The IM component LptB2FG comprises an ATP-binding cassette (ABC) transporter, which powers the transport of LPS across the bridge. The cytoplasmic LptB dimer binds and hydrolyses ATP and the transmembrane (TM) domains of LptF and LptG create a cavity to accommodate LPS. LptB2 constitutes the cytoplasmic NBD dimer and the six TM helices of LptF and LptG (F_TM1-TM6 and G_TM1-TM6) constitute two TMDs that are arranged to form a central cavity with two surface gaps between TM1F and TM5G and TM1G and TM5F termed as lateral gates. To understand the mechanisms of how LptB2FGC recognises and acts to transport LPS, we obtained high-resolution cryo-electron microscopy (cryo-EM) structures of LptB2FGC complexed with substrate LPS or ATP analogue β-γ-imidoadenosine 5′-triphosphate (AMP-PNP).

The cryo-EM structure of sfLptB2FGC was determined to 3.1 Å resolution. However, due to possible flexibility, we are unable to see clear density for the periplasmic domain of LptC. In our structure, residues M1, R5, I9, L12, V16, M19 and N23 from the TM helix of LptC interact with residues Q293, L300, L305, L304, L307, L311 and T314 from the TM5 of LptF, respectively. In contrast, only G21 from the TM helix of LptC interacts with V36 of TM1 of LptG. Comparing to the sfLptB2FG LPS-bound structure, the presence of the TM helix of LptC makes the lateral gate TM1G/TM5F of sfLptB2FGC structure much widely opened, along with the neighbouring TM2 and TM3 of LptG and TM4 and TM6 of LptF moved outward, resulting an enlarged central cavity. In contrast to the two recent publications, a density for LPS is identified in the cavity of sfLptB2FGC with all features visible as in the sfLptB2FG structure except the inner core of the LPS. Interestingly, the LPS molecule trapped in the cavity of sfLptB2FGC is about 7.3 Å away from that of sfLptB2FG structure referring to the position of the 1′-phosphate group. The LPS molecule in the sfLptB2FGC structure positions in proximity to LptG with kinked acyl tails rather than drooped as seen in the sfLptB2FG structure. In the cavity of sfLptB2FGC, we can also see that hydrophobic residues L17 and M24 from the TM helix of LptC interact with the bound LPS, suggesting that the TM helix of LptC is also involved in LPS recognition. The number of residues from the TM helices of LptF and LptG that have been shown to interact with LPS in the enlarged cavity of sfLptB2FGC are greatly reduced compared to the structure of sfLptB2FG.

>[2x]MATLTAKNLAKAYKGRRVVEDVSLTVNSGEIVGLLGPNGAGKTTTFYMVVGIVPRDAGNIIIDDDDISLLPLHARARRGIGYLPQEASIFRRLSVYDNLMAVLQIRDDLSAEQREDRANELMEEFHIEHLRDSMGQSLSGGERRRVEIARALAANPKFILLDEPFAGVDPISVIDIKRIIEHLRDSGLGVLITDHNVRETLAVCERAYIVSQGHLIAHGTPTEILQDEHVKRVYLGEDFRL;> MSKARRWVIIVLSLAVLVMIGINMAEKDDTAQVVVNNNDPTYKSEHTDTLVYNPEGALSYRLIAQHVEYYSDQAVSWFTQPVLTTFDKDKIPTWSVKADKAKLTNDRMLYLYGHVEVNALVPDSQLRRITTDNAQINLVTQDVTSEDLVTLYGTTFNSSGLKMRGNLRSKNAELIEKVRTSYEIQNKQTQP;> MIIIRYLVRETLKSQLAILFILLLIFFCQKLVRILGAAVDGDIPANLVLSLLGLGVPEMAQLILPLSLFLGLLMTLGKLYTESEITVMHACGLSKAVLVKAAMILAVFTAIVAAVNVMWAGPWSSRHQDEVLAEAKANPGMAALAQGQFQQATNGSSVLFIESVDGSDFKDVFLAQIRPKGNARPSVVVADSGHLTQLRDGSQVVTLNQGTRFEGTALLRDFRITDFQDYQAIIGHQAVALDPNDTDQMDMRTLWNTDTDRARAELNWRITLVVTVFMMALMVVPLSVVNPRQGRVLSMLPAMLLYLLFFLIQTSLKSNGGKGKLDPTLWMWTVNLIYLALAIVLNLWDTVPVRRLRASFSRKGAV;> MQPFGVLDRYIGKTIFTTIMMTLFMLVSLSGIIKFVDQLKKAGQGSYDALGAGMYTLLSVPKDVQIFFPMAALLGALLGLGMLAQRSELVVMQASGFTRMQVALSVMKTAIPLVLLTMAIGEWVAPQGEQMARNYRAQAMYGGSLLSTQQGLWAKDGNNFVYIERVKGDEVLGGISIYAFNENRRLQSVRYAATAKFDPEHKVWRLSQVDESDLTNPKQITGSQTVSGTWKTDLTPDKLGVVALDPDALSISGLHNYVKYLKSSGQDAGRYQLNMWSKIFQPLSVAVMMLMALSFIFGPLRSVPMGVRVVTGISFGFVFYVLDQIFGPLTLVYGIPPIIGALLPSASFFLISLWLLMRKS10-FORMYL-5,8,10-TRIDEAZAFOLIC 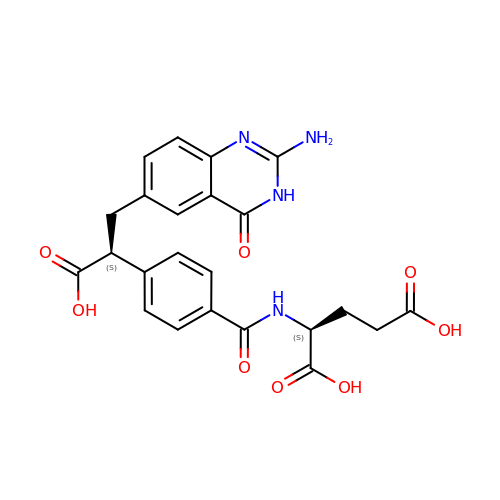ACID | C23 H22 N4 O8 | DAOQLLQRJAXMGY-YOEHRIQHSA-N1-[4-(4-hydroxyphenyl)piperazin-1-yl]ethanone | C12 H16 N2 O2 | 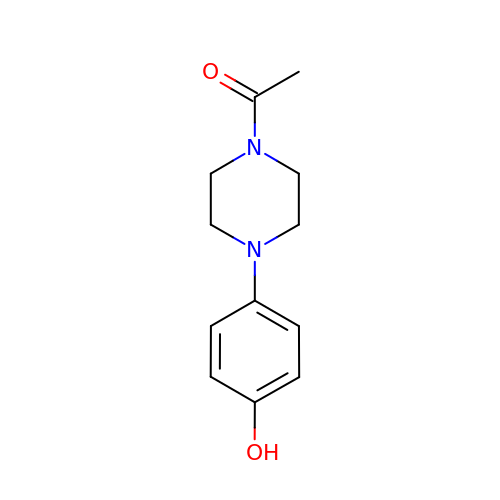AGVNLFCRZULMKK-UHFFFAOYSA-N> VADTDDTATLRYPGG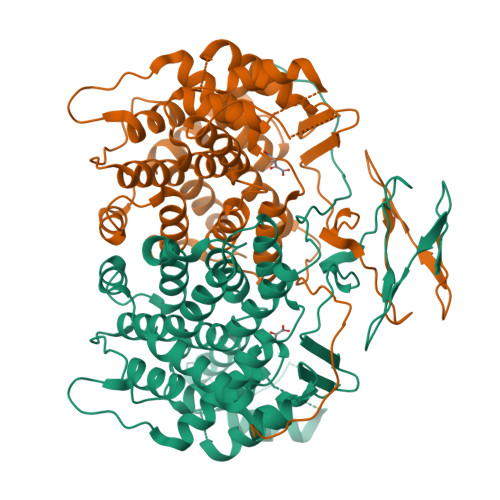EIDLQIVHATEGADGIALGPLLAKTGHTTFDVGFANTAAAKSSITYIDGDAGILRYRGYPIDQLAEKSTFIEVCYLLIYGELPDTDQLAQFTGRIQRHTMLHEDLKRFFDGFPRNAHPMPVLSSVVNALSAYYQDALDPMDNGQVELSTIRLLAKLPTIAAYAYKKSVGQPFLYPDNSLTLVENFLRLTFGFPAEPYQADPEVVRALDMLFILHADHEQNCSTSTVRLVGSSRANLFTSISGGINALWGPLHGGANQAVLEMLEGIRDSGDDVSEFVRKVKNREAGVKLMGFGHRVYKNYDPRARIVKEQADKILAKLGGDDSLLGIAKELEEAALTDDYFIERKLYPNVDFYTGLIYRALGFPTRMFTVLFALGRLPGWIAHWREMHDEGDSKIGRPRQIYTGYTERDYVTIDAR> SPSAEACGYSDRVAQLTLGNSTITTQEAANICVAYGCWPAKLSDTDATSVDKPTEPGVSADRFYTLRSKPWQADSKGWYWKLPDALNNTGMFGQNAQFHYLYRGGWAVHVQCNATKFHQGTLLVLAIPEHQIATQEQPAFDRTMPGSEGGTFQEPFWLEDGTSLGNSLIYPHQWI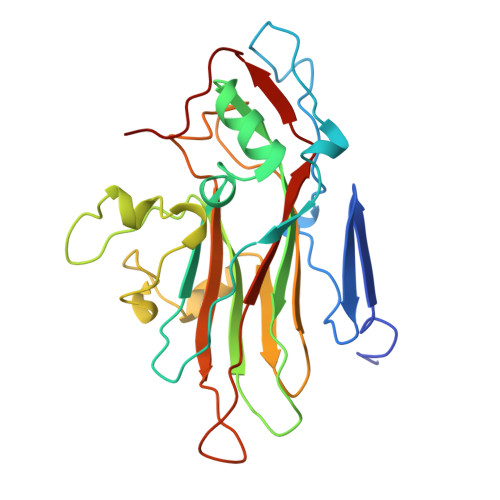NLRTNNSATLILPYVNAIPMDSAIRHSNWTLAIIPVAPLKYAAETTPLVPITVTIAPMETEYNGLRRAIASNQ> GDPVEDIIHDALGNTARRAISGATNVESAADTTPSSHRLETGRVPALQAAETGATSNATDENMIETRCVINRNGVLETTINHFFSRSGLVGVVNLTDGGDTTGYATWDIDIMGFVQLRRKCEMFTYMRFNAEFTFVTTTKSGEARPYMLQYMYVPPGAPKPTGRDAFQWQTATNPSVFVKLTDPPAQVSVPFMSPASAYQWFYDGYPTFGQHPETSNTTYGLCPNNMMGTFAVRVVSREASQLKLQTRVYMKLKHVRAWVPRPIRSQPYLLKNFPNYDSSKITNSARDRSSIKQANM;> MGAQVSTQKSGSHETGNVATGGSTINFTNINYYKDSYAASATRQDFTQDPKKFTQPVLDSIRELSAPLNSPSVEACGYSDRVAQLTVGNSSITTQEAANIVLAYGEWPEYCPDTDATAVDKPTRPDVSVNRFYTLDSKMWQENSTGWYWKFPDVLNKTGVFGQNAQFHYLYRSGFCLHVQCNASKFHQGALLVAVIPEFVIAGRGSNTKPNEAPHPGFTTTFPGTTGATFHDPYVLDSGVPLSQALIYPHQWVNLRTNNCATVIVPYINAVPFDSAINHSNFGLVVVPVSPLKYSSGATTAIPITITIAPLNSEFGGLRQAVSQ;> GIPAELRPGTNQFLTTDDDTAAPILPGFTPTPTIHIPGEVHSLLELCRVETILEVNNTTEATGLTRLLIPVSSQNKADELCAAFMVDPGRIGPWQSTLVGQICRYYTQWSGSLKVTFMFTGSFMATGKMLVAYSPPGSAQPANRETAMLGTHVIWDFGLQSSVSLVIPWISNTHFRTAKTGGNYDYYTAGVVTLWYQTNYVVPPETPGEAYIIAMGAAQDNFTLKICKDTDEVTQQAVLQ

Coxsackievirus A10 (CV-A10) belongs to the enterovirus genus in the Picornaviridae family. The virus is considered one of the major causative agents of hand, foot, and mouth disease (HFMD), which is highly infectious and affects millions of young children annually. In general, enteroviral capsids are composed of 60 copies of biological protomers that are arranged in a pseudo-T = 3 icosahedral symmetry. Each protomer consists of four capsid proteins, including VP1, VP2, VP3, and VP4.

Human enteroviruses from cell cultures often exist in two forms: one is infectious mature virion (also termed “F-particle”), which contains viral RNA genome, and the other is non-infectious native empty particle (NEP) (also termed “E-particle”) without viral RNA genome. In the NEP map, some surface-exposed loops, such as the GH loops of VP1 and VP3, are unresolved; additionally, residues 1–96, 112–123, and 321–324 of VP0, 1–72 and 297 of VP1, and 176–182 of VP3 are also missing in this map. According to our maps, NEP is slightly expanded compared with mature virion (157 vs. 152 Å in radius, ~3% expansion). Compared with the mature virus, NEP exhibits a 4.8° counter-clockwise rotation of the protomeric building block (VP1, VP0, and VP3) pivoting about the corner of VP3 at the icosahedral three-fold axis, and the VP1 was pushed away from quasi-three-fold axis region exhibiting a 6 Å shift towards the five-fold axis, leading to enlarged spacing between protomers. Specifically, the two-fold axis channel is markedly opened in the NEP than in mature virion (indicated by dashed rectangles in Fig. 2e, f). No density corresponding to the pocket factor was observed in the CV-A10 NEP map. In fact, the hydrophobic pocket is collapsed in the NEP compared with that in the mature virion. The volume of the pocket is significantly reduced because four residues (Ile109, Val191, Met228, and Phe231 of VP1) move inward, making it impossible to accommodate the pocket factor.(3R)-3-ethyl-N-[(4-methylphenyl)sulfonyl]-L-aspartic acid | C13 H17 N O6 S | 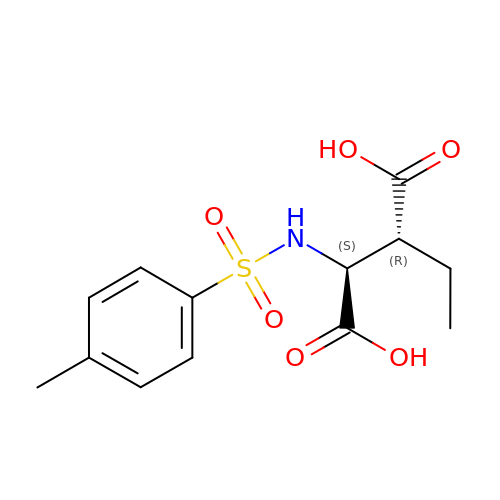KPHLTCNXHCHMOW-MNOVXSKESA-N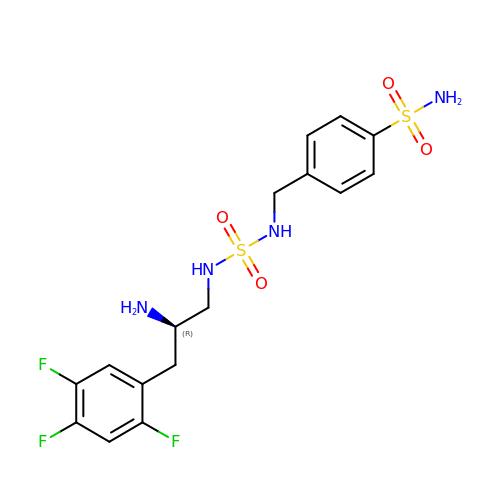4-[({[(2R)-2-amino-3-(2,4,5-trifluorophenyl)propyl]sulfamoyl}amino)methyl]benzenesulfonamide | C16 H19 F3 N4 O4 S2 | DJEOZKIXGQHLQG-GFCCVEGCSA-N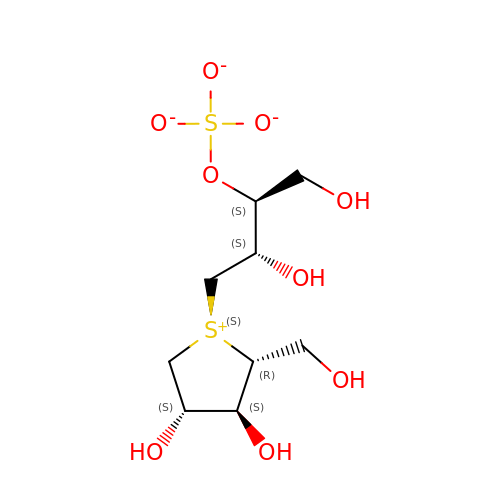1,4-DIDEOXY-1,4-[[2S,3S)-2,4-DIHYDROXY-3-(SULFOXY)BUTYL]EPISULFONIUMYLIDENE]-D-ARABINITOL INNER SALT | C9 H18 O9 S2 | NYHLFUZUGSMDBR-YRPOCYRVSA-L> KGGAKR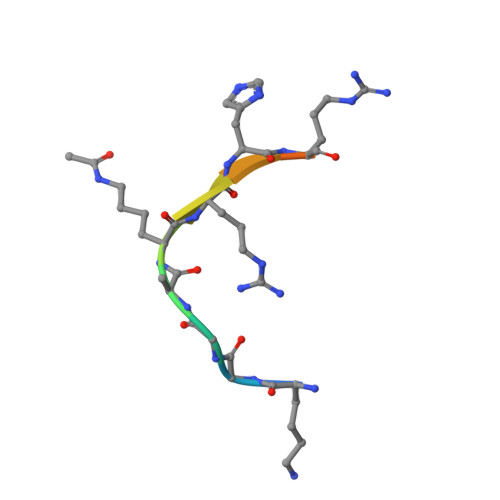HRKIL>RVVCREASHAGSWYTASGPQLNAQLEGWLSQVQSTKRPARAIIAPHAGYTYCGSCAAHAYKQVDPSITRRIFILGPSHHVPLSRCALSSVDIYRTPLYDLRIDQKIYGELWKTGMFERMSLQTDEDEHSIEMHLPYTAKAMESHKDEFTIIPVLVGALSESKEQEFGKLFSKYLADPSNLFVVSSDFCHWGQRFRYSYYDESQGEIYRSIEHLDKMGMSIIEQLDPVSFSNYLKKYHNTICGRHPIGVLLNAITELQKNGMNMSFSFLNYAQSSQCRNWQDSSVSYAAGALTVH[4x]

Mediator of ERBB2-driven cell motility 1 (MEMO1) is an evolutionary conserved protein implicated in many biological processes; however, its primary molecular function remains unknown. MEMO1 is a highly conserved protein found in the cytosol of eukaryotic cells from yeast to humans. We conclude that MEMO1 is an iron-binding protein that modulates iron homeostasis in cancer cells. Our work reveals that the iron coordination mode in MEMO1 is very similar to that of iron-containing extradiol dioxygenases, which also display a similar structural fold.

To reveal the binding mode of each metal, we have crystallized MEMO1 in the presence of iron or copper under the conditions similar to those used previously for solving the structure of the metal-free protein. To prevent metal oxidation, MEMO1 crystallization with iron (II) or copper (I) was set up in an anaerobic chamber and the plates were incubated under argon, while the crystals were growing. When MEMO1 was crystallized in the presence of copper, the copper atom bound at the same site, and was coordinated by the same residues as iron. The protein fold of both metal-bound forms of MEMO1 is essentially identical to the metal-free structure, with RMSD for α-carbons of the superimposed structures being less than 0.17 Å. In the absence of iron, we have also observed binding of copper (added as Cu(I)) to MEMO1 at a molar ratio of copper to protein of approximately 0.4. Copper (I) binding was also detected by ITC, with an estimated Kd of about 3×10–6 M. Thus, metal coordination in MEMO1 is achieved by H49, H81, and C244, while H192 and D189 do not participate in metal binding in MEMO1. Therefore, in the absence of specific copper loading mechanisms for MEMO1, it is likely to predominantly bind iron in the cytosol of the living cells, even though copper binding can be observed in vitro. Still, consistent with the previous reports, MEMO1 may bind copper under oxidative conditions in a specific local environment within the cell, and it is tempting to speculate that metal-binding change may trigger a switch between different MEMO1 activities in the cell.> SNEPLSSTEAPSRPMDVVTAPNQADPRAYPFAPADLVVEILDLVQQAS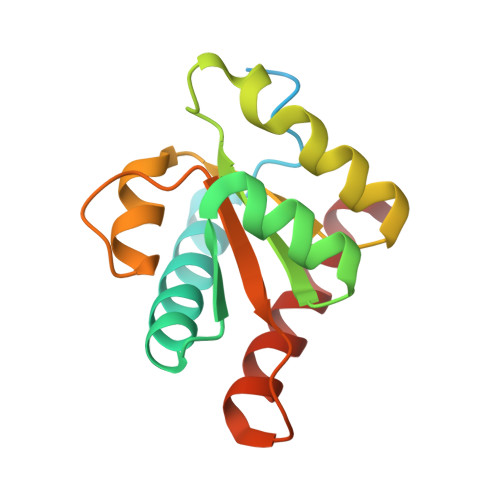HYKQIKKGLNEVLKSMNRGLAEFVVLAADTQPLEILLSAPLVAEDKAVPYVFVPSKAALGRACGVSRPVIACAVLRADMSQLRNQITALRTKIEQLLL>[4x]GFPIPDPYCWDISFRTFYTIIDDEHKTLFNGILLLSQADNADH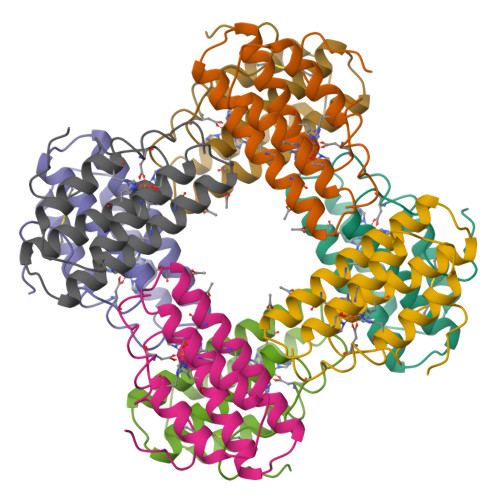LNELRRCTGKHFLNEQQLMQASQYAGYAEHKKAHDDFIHKLDTWDGDVTYAKNWLVNHIKTIDFKYRGKI1,3-DIHYDROXYPROPAN-2-YL (Z)-TETRADEC-7-ENOATE 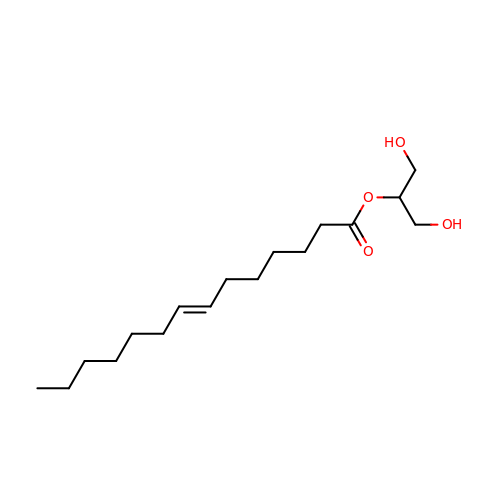| C17 H32 O4 | SSMGVWSPWWDBRB-FPLPWBNLSA-N>[8x]MAKKRASGVLMHITSL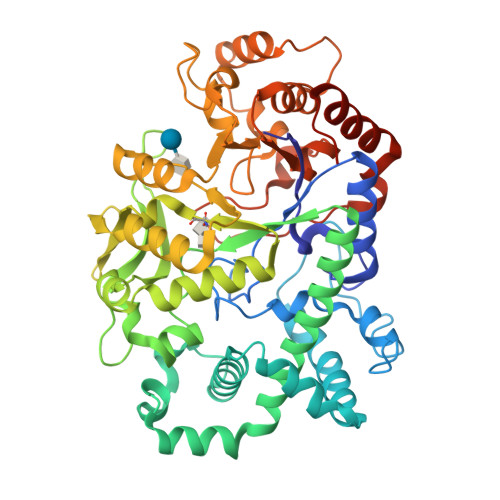PGDLGIGTFGREAYAFVDFLVETDQKFWQILPLTTTSFGDSPYQSFSAVAGNTHLIDFDLLTLEGFISKDDYQNISFGQDPEVVDYAGLFEKRRPVLEKAVKNFLKEERATRMLSDFLQEEKWVTDFAEFMAIKEHFGNKALQEWDDKAIIRREEEALAGYRQKLSEVIKYHEVTQYFFYKQWFELKEYANDKGIQIIGDMPIYVSADSVEVWTMPELFKLDRDKQPLAIAGVPADDFSDDGQLWGNPIYNWDYHKESDFDWWIYRIQSGVKMYDYLRIDHFKGFSDYWEIRGDYQTANDGSWQPAPGPELFATIKEKLGDLPIIAENLGYIDERAERLLAGTGFPGMKIMEFGFYDTTGNSIDIPHNYTENTIAYAGTHDNEVINGWFENLTVEQKAYAENYMRRLPNEPITETVLRTLYATVSQTTITCMQDLLDKPADSRMNMPNTVGGNWQWRMRKEDLTENRKAFLKEITTIYNRGNKLEHHHHHH> QWALEDFEIGRPLGKGKFGNVYLAREKQRKFILALKVLFKAQLEKAGVEHQLRREVEIQSHLRHPNI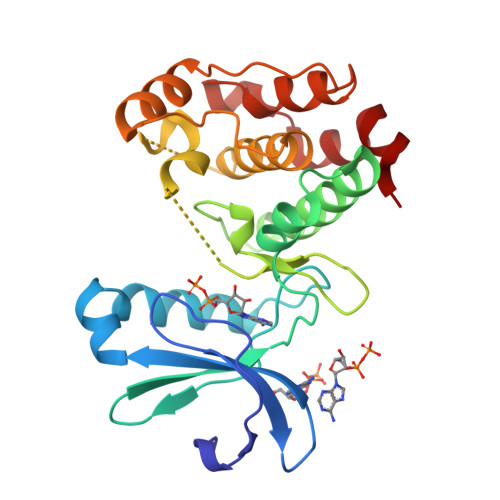LRLYGYFHDATRVYLILEYAPLGTVYRELQKLSKFDEQRTATYITELANALSYCHSKRVIHRDIKPENLLLGSAGELKIADFGWSVHAPSSRRTTLCGTLDYLPPEMIEGRMHDEKVDLWSLGVLCYEFLVGKPPFEANTYQETYKRISRVEFTFPDFVTEGARDLISRLLKHNPSQRPMLREVLEHPWITANSS> MGSSHHHHHHSSGLVPRGSHPSLRTQPSLYSGPFPFYRRPSELGCFSLDAQRQYHGDARALRYYSPPPINGPGPDFDLRDGYPDRYQPRDEEVQERLDHLLRWVLEHRNQLEGGPGWLAGATVTWRGHLTKLLTTPYERQEGWQLAASRFQGTLYLSEVETPAARAQRLARPPLLRELMYMGYKFEQYMCADKPGGSPDPSGEVNTNVAYCSVLRSRLGNHPLLFSGEVDCLNPQAPCTQPPSCYVELKTSKEMHSPGQWRSFYRHKLLKWWAQSFLPGVPHVVAGFRNPEGFVCSLKTFPTMEMFENVRNDREGWNPSVCMNFCAAFLSFAQSTVVQDDPRLVHLFSWEPGGPVTVSVHRDAPYAFLPSWYVETMTQ

In eukaryotes, the DXO/Rai1 family of enzymes removes numerous 5′-end RNA modifications, thereby regulating RNA turnover. Mouse DXO catalyzes the elimination of incomplete 5′-end caps (including pyrophosphate) and the non-canonical NAD+ cap on mRNAs, and possesses distributive 5′-3′ exoribonuclease activity toward 5′-monophosphate (5′-PO4) RNA. Six conserved sequence motifs (I–VI) form the active site which is located within a deep pocket, and several residues in these motifs bind divalent cations for catalysis. Here, we demonstrate that DXO also catalyzes the hydrolysis of RNAs bearing a 5′-hydroxyl group (5′-OH RNA).

To understand the molecular basis for the catalytic activity of DXO toward 5′-OH RNA, we determined the crystal structure of wild-type mouse DXO in complex with a 5′-OH hexa-nucleotide non-hydrolyzable RNA substrate mimic, OH-U(S)6. DXO crystals were soaked with OH-U(S)6 RNA and with calcium as the divalent cation to further block hydrolysis. We observed good electron density for four nucleotides of the OH-U(S)6 RNA and a calcium ion in the complex with DXO. There is electron density for a calcium ion bound to the active site residues (Asp236, Glu253 and Glu192), and this density is not observed in crystals not soaked with calcium. However, the calcium ion contacts the phosphorothioate group between the second and third nucleotides of this RNA instead of between the first and second as was observed with pU(S)6 (15). This suggests that the scissile phosphate of this 5′-OH RNA is located between its second and third nucleotides, and more importantly, it predicts that DXO generates a 5′-OH dinucleotide as the first product of the hydrolysis. The U0 base has π stacking interactions with the mostly conserved Trp131 side chain, and it also makes three hydrogen-bonding contacts: to the backbone carbonyl of Arg102 and the side chain of His105 directly and to the backbone amide of His105 through a water molecule. The 5′-OH moiety itself is intimately packed against the base of U(S)1. The presence of a phosphate here would make it impossible to adopt this conformation, which may account for why 5′-PO4 RNA cannot bind in this manner. In addition, the U(S)1 base is in the syn configuration in OH-U(S)6 RNA, while it is anti in pU(S)6.>[4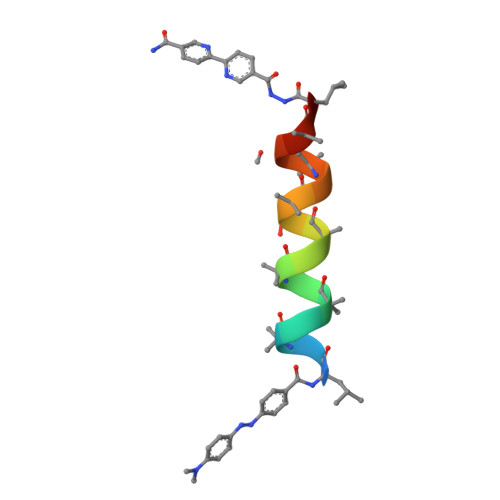x]XLAAAAAALAAALAQALX> IPVIEPLFTKVTEDIPGAEGPVFDKNGDFYIVAPEVEVNGKPAGEILRIDLKTGKKTVICKPEVNGYGGIPAGCQCDRDANQLFVADMRLGLLVVQTDGTFEEIAKKDSEGRRMQGCNDCAFDYEGNLWITAPAGEVAPADYTRSMQEKFGSIYCFTTDGQMIQVDTAFQFPDGIAVRHMNDGRPYQLIVAETPTKKLWSYDIKGPAKIENKKVWGHIPGTHEGGADGMDFDEDNNLLVANWGSSHIEVFGPDGGQPKMRIRCPFEKPSNLHFKPQTKTIFVTEHENNA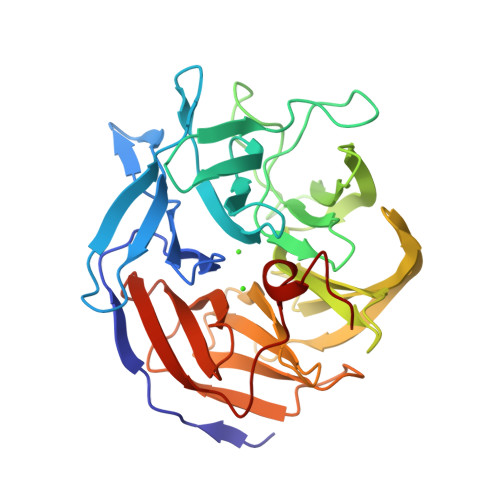VWKFEWQRNGKKQYCETLKFGIF The cell-death-inducing DFF45-like effector (CIDE) domain is a protein-interaction module comprising ∼80 amino acids and was initially identified in several apoptotic nucleases and their regulators. DREP3 is a CIDE-domain-containing protein in Drosophila and has been suggested to be a regulator of nucleases. Unlike proteins harbouring the CIDE domain at the N-terminus, the DREP3 CIDE domain is located in the middle of the protein.

To further understand this dynamic protein-interaction module, we obtained a crystal of the DREP3 CIDE domain which had a calculated Matthews coefficient (V M) of 2.76 Å3 Da−1, corresponding to a solvent content of 55.43%, and solved the structure at a resolution of 3.0 Å. The final model contained residues 117–193 for all nine molecules.

>[9x]FAQLDNSKPFKIKDITRNIRKAVVATTISEIRTKVSLKFERAQRRIHLDCDGTEVDDEEYFSTLEPNAELIAVFPGEQWRDPSD Acid sphingomyelinase (ASMase, ASM, SMPD1) is an enzyme found in lysosomes and in the extracellular space where it catalyses the conversion of sphingomyelin, a major component of membranes, into ceramide and phosphocholine. ASMase consists of an N-terminal saposin domain and a C-terminal catalytic domain. To gain insight into the molecular mechanism of ASMase function and the interplay between its domains, we determined crystal structures of the full-length protein from mouse that reveal a conformational flexibility of the saposin domain. In one conformation, the saposin domain adopts a globular closed form independent of the catalytic domain, while in the other conformation, it assumes an open V-shaped fold that establishes an extended interface with the catalytic domain.

As observed with other saposins, ASMasesap adopts either a closed or open conformation depending on environmental conditions. By contrast, the open form of ASMasesap assumes a V-shaped conformation with its hydrophobic core exposed and its position shifted on ASMasecat such that one face of helix α3 forms an extensive 1,318 Å2, hydrophobic interface with ASMasecat. To assess the significance of this interface for sphingomyelin hydrolysis, we measured the activity of interface mutants on anionic liposomes containing sphingomyelin at acidic pH to mimic the lysosomal environment. Deletion of ASMasesap almost completely abrogated activity and six interface mutants substantially reduced activity, verifying that both the saposin domain and the interface are required for membrane sphingomyelin hydrolysis. The interface presumably stabilizes the open conformation of ASMasesap, allowing it to dock onto membrane surfaces, and possibly deliver lipids to the active site. Closer examination of the interface revealed direct contacts between ASMasesap and active site loops of ASMasecat, hinting at a coupling between lipid binding, interface formation and catalytic activity. The structure of isolated ASMasecat is unchanged relative to the catalytic domain in the open form full-length protein, but analysis of their crystal temperature factors indicated that interface formation reduces catalytic loop dynamics. This suggests that the interface is important not only for stabilizing open ASMasesap for membrane docking, but also for stabilizing ASMasecat and activating catalysis. The location on open ASMasesap responsible for membrane lipid docking under physiological conditions likely includes its hydrophobic surface, which in the crystal is buried by a symmetry-related saposin domain reminiscent of the ‘handshake' clasp observed in saposin B dimers. In the presence of anionic membranes, open ASMasesap becomes prevalent, docks onto the membrane surface and concomitantly forms an interface with the catalytic domain activating it for sphingomyelin hydrolysis.

>DRHHHHHHKLNLTCPACKVLFTALNHGLKKEPNVARVGSVAIKICKMLNIAPLDVCQSAVHLFEDDVVEVWTRSVLSPSEACGLLLGSSCGHWDIFSTWNISLPSVPKPPPKPPSPPAPGAPVSRVLFLTDLHWDHEYLEGTDPYCADPLCCRRGSGWPPNSQKGAGFWGEYSKCDLPLRTLESLLKGLGPAGPFEMVYWTGDIPAHDVWQQSRQDQLRALTTITDLVRKFLGPVPVYPAVGNHESTPVNGFPPPFIKGNQSSQWLYEAMAKAWEPWLPADALHTLRIGGFYALTPRPGLRLISLNMNFCSRENFWLLINSTDPAGQLQWLVEELQAAENRGDKVHIIGHIPPGHCLKSWSWNYYKIIARYENTLAGQFFGHTHVDEFEIFYDEETLSRPLAVAFLAPSATTFINLNPGYRVYQIDGNYPGSSHVVLDHETYILNLTQANAAGGTPSWKRLYRARETYGLPDAMPASWHNLVYRMRDDEQLFQTFWFLYHKGHPPSEPCGTPCRLATLCAQLSARADSPALCRHLMPN[2x]> MVSVSEIRKAQRAEGPATILAIGTANPANCVEQSTYPDFYFKITNSEHKTELKEKFQRMCDKSMIKRRYMYLTEEILKENPNVCEYMAPSLDARQDMVVVEVPRLGKEAAVKAIKEWGQPKSKITHLIVCTTSGVDMPGADYQLTKLLGLRPYVKRYMMYQQGAFAGG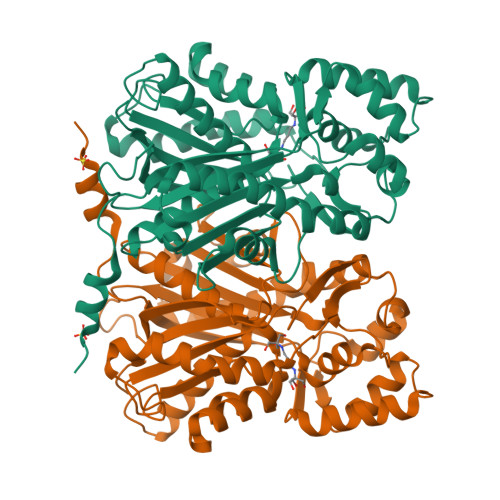TVLRLAKDLAENNKGARVLVVCSEVTAVTFRGPSDTHLDSLVGQALFGDGAAALIVGSDPVPEIEKPIFEMVWTAQTIAPDSEGAIDGHLREAGLTFHLLKDVPGIVSKNITKALVEAFEPLGISDYNSIFWIAHPGGPAILDQVEQKLALKPEKMNATREVLSEYGNMSSACVLFILDEMRKKSTQNGLKTTGEGLEWGVLFGFGPGLTIETVVLRSVAI> GDPIADMIDQTVNNQVNRSLTALQVLPTAANTEASSHRLGTGVVPALQAAETGASSNASDKNLIETRCVLNHHSTQETAIGNFFSRAGLVSIITMPTMGTQNTDGYANWDIDLMGYAQLRRKCELFTYMRFDAEFTFVVAKPNGELVPQLLQYMYVPPGAPKPTSRDSFAWQTATNPSVFVKMTDPPAQVSVPFMSPASAYQWFYDGYPTFGEHLQANDLDYGQCPNNMMGTFSIRTVGTKKSPHSITLRVYMRIKHVRAWIPRPLRNQPYLFKTNPNYKGNDIKCTSTSRDKITTL;> SPSAEACGYSDRVAQLTIGNSTITTQEAANIVIAYGEWPEYCPDTDATAVDKPTRPDVSVNRFFTLDTKSWAKDSKGWYWKFPDVLTEVGVFGQNAQFHYLYRSGFCVHVQCNASKFHQGALLVAVLPEYVLGTIAGGTGNENSHPPYATTQPGQVGAVLTHPYVLDAGIPLSQLTVCPHQWINLRTNNCATIIVPYMNTVPFDSALNHCNFGLLVIPVVPLDFNAGATSEIPITVTIAPMCAEFAGLRQAVKQ;> GIPTELKPGTNQFLTTDDGVSAPILPGFHPTPPIHIPGEVRNLLEICRVETILEVNNLKTNETTPMQRLCFPVSVQSKTGELCAAFRADPGRDGPWQSTILGQLCRYYTQWSGSLEVTFMFAGSFMATGKMLIAYTPPGGSVPADRITAMLGTHVIWDFGLQSSVTLVVPWISNTHYRAHARAGYFDYYTTGIIT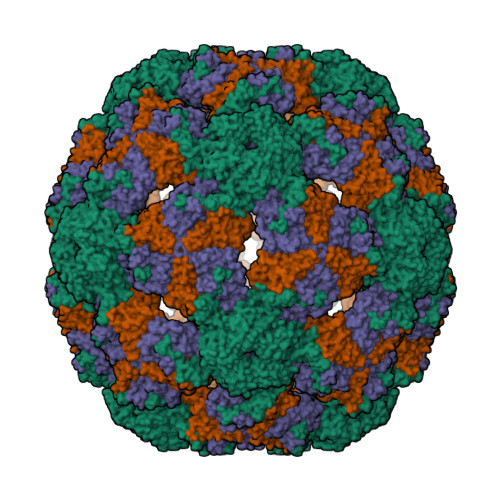IWYQTNYVVPIGAPTTAYIVALAAAQDNFTMKLCKDTEDIEQTANIQ>MTMMTATQALSVNPATGQTLAAMPWANAQEIEHALSLAASGFKKWKMTSVAQRAQTLRDIGQALRAHAEEMAQCITREMGKPIKQARAEVTKSAALCDWYAEHGPAMLNPEPTLVENQQAVIEYRPLGVILAIMPWNFPLWQVLRGAVPILLAGNSYLLKHAPNVTGCAQMIARILAEAGTPAGVYGWVNANNEGVSQMINDPRIAAVTVTGSVRAGAAIGAQAGAALKKCVLELGGSDPFIVLNDADLELAVKAAVAGRYQNTGQVCAAAKRFIVEEGIAQAFTDRFVAAAAALKMGDPLVEENDLGPMARFDLRDELHQQVQASVAEGARLLLGGEKIAGEGNYYAATVLADVTPD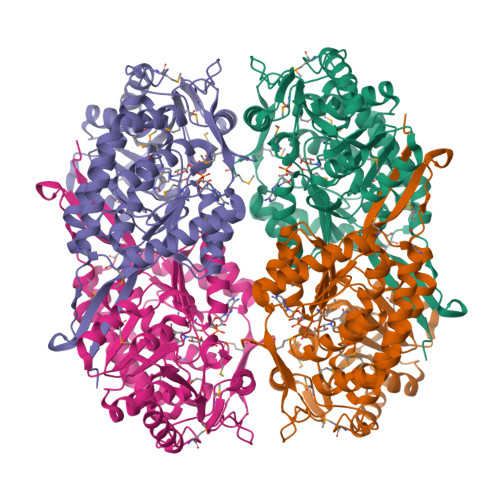MTAFRQELFGPVAAITVAKDAAHALALANDSEFGLSATIFTADDTLAAEMAARLECGGVFINGYSASDARVAFGGVKKSGFGRELSHFGLHEFCNVQTVWKNRV[4x]>MASCRSSRKPALTPARATVIIMLIMTTTLTAT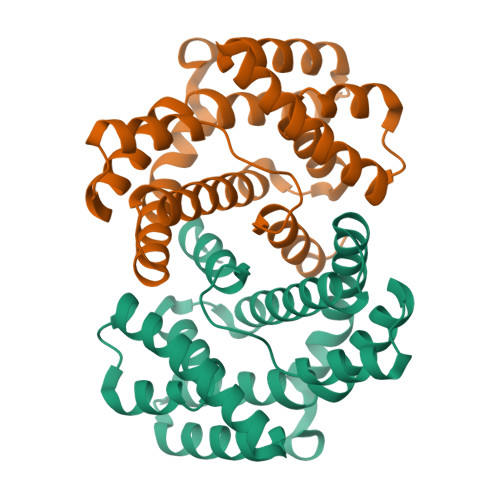SMSTAEQRLRLMQLASSNLPVGGYSWSQGLEWAVEAGWVPDVAAFERWQRRQMTEGFFTVDLPLFARLYRACEQGDIAAAQRWTAYLLACRETRELREEERNRGAAFARLLSDWQPDCPPPWRSLCQQSQLAGMAWLGVRWRIALPEMALSLGYSWIESAVMAGVKLVPFGQQAAQQLILRLCDHYAAEMPRALAAPDGDIGSATPLAAIASARHETQYSRLFRS[4x]>[2x]HHHHHHSAALEVLFQGPGMEVSTNPSSNIDPGDYVEMNDSITHLPSKVVIQDITMELHCPLCNDWFRDPLMLSCGHNFCEACIQDFWRLQAKETFCPECKM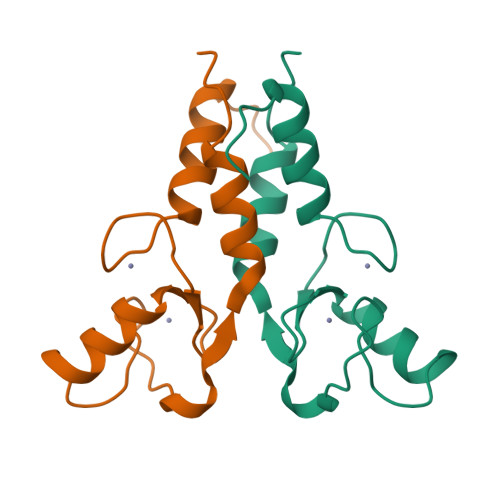LCQYNNCTFNPVLDKLVEKIKKLPLLK>ARPCIPKSFGYSSVVCVCNATYCDSFDPPTFPALGTFSRYESTRSGRRMELSMGPIQANHTGTGLLLTLQPEQKFQKVKGFGGAMTDAAALNILALSPPAQNLLLKSYFSEEGIGYNIIRVPMASCDFSIRTYTYADTPDDFQLHNFSLPEEDTKLKIPLIHRALQLAQRPVSLLASPWTSPTWLKTNGAVNGKGSLKGQPGDIYHQTWARYFVKFLDAYAEHKLQFWAVTAENEPSAGLLSGYPFQCLGFTPEHQRDFIAR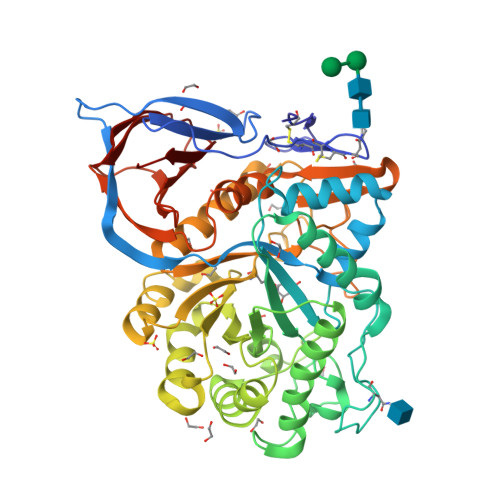DLGPTLANSTHHNVRLLMLDDQRLLLPHWAKVVLTDPEAAKYVHGIAVHWYLDFLAPAKATLGETHRLFPNTMLFASEACVGSKFWEQSVRLGSWDRGMQYSHSIITNLLYHVVGWTDWNLALNPEGGPNWVRNFVDSPIIVDITKDTFYKQPMFYHLGHFSKFIPEGSQRVGLVASQKNDLDAVALMHPDGSAVVVVLNRSSKDVPLTIKDPAVGFLETISPGYSIHTYLWRRQ[2x]2,6,11-trimethoxy-4,7,9-tris(oxidanyl)-1,12-bis[(2R)-2-oxidanylpropyl]perylene-3,10-dione | C29 H28 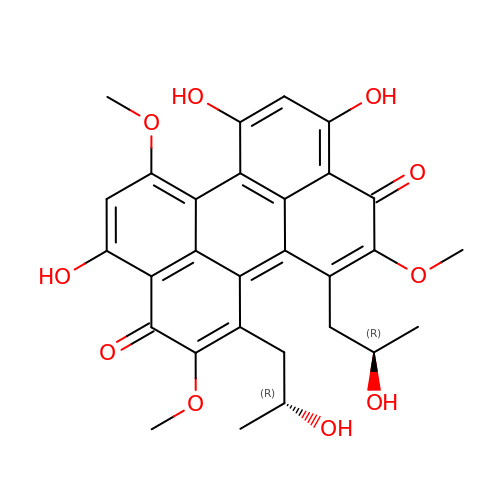O10 | SZXDWEFJNLPCTA-GHMZBOCLSA-N>[2x]MDHLPIFCQLRDRDCLIVGGGDVAERKARLLLEAGARLTVNALTFIPQFTVWANEGMLTLVEGPFDETLLDSCWLAIAATDDDTVNQRVSDAAESRRIFCNVVDAPKAASFIMPSIIDRSPLMVAVSAGGTSPVLARLLREKLESLLPQHLGQVARYAGQLRARVKKQFATMGERRRFWEKFFVNDRLAQSLANADEKAVNATTERLFSEPLDHRGEVVLVGAGPGDAGLLTLKGLQQIQQADIVVYDRLVSDDIMNLVRADADRVFVGKRAGYHCVPQEEINQILLREAQKGKRVVRLKGGDPFIFGRGGEELETLCHAGIPFSVVPGITAASGCSAYSGIPLTHRDYAQSVRLVTGHLKTGGELDWENLAAEKQTLVFYMGLNQAATIQEKLIAFGMQADMPVALVENGTSVKQRVVHGVLTQLGELAQQVESPALIIVGRVVALRDKLNWFSNH

Siroheme is the modified isobacteriochlorin tetrapyrrole used by siroheme-dependent sulfite and nitrite reductases (SiR/NiRs) in catalyzing the six-electron reduction of sulfite to sulfide or nitrite to ammonia. CysG is encoded by a gene fusion between a C-terminal SUMT (CysGA) and an N-terminal bifunctional dehydrogenase/ferrochelatase (CysGB). The N-terminal enzyme module, CysGB, is a three-domain bifunctional dehydrogenase/ATP-independent class III ferrochelatase12 that performs the final two steps of siroheme biosynthesis. The C-terminal enzyme module, CysGA, is homologous to a well-studied class of SAM-dependent uro’gen III methyltransferases (SUMTs) that catalyzes the methylations to generate precorrin-210,13.

R260, which binds ring C C12 acetyl, and R261, which does not directly interact with carboxylate but contributes to the positively charged pocket that captures ring B, are part of the CysGA SUMT module. To test whether or not their contributions are essential for tetrapyrrole binding, we individually altered each to an alanine and tested the variants’ activities for dehydrogenase or chelatase activity. Both the R260A and R261A variants complement a cysG deficiency in E. coli grown on minimal media where SO42− is the sole sulfur source. The R261A variant has ~40-fold lower dehydrogenase activity and 20-fold lower chelatase activity. We next determined the X-ray crystal structures of the variants to test whether these alterations changed the relationship between the enzyme modules or their overall structure. Both R260A and R261A structures are similar to CysG and have a low root-mean-square deviation (RMSD) when aligned against Met8p14. R261 does not make a formal interaction with the tetrapyrrole, although it does contribute to the charged pocket that binds the carboxylates from ring B, so it is not surprising that removing the large, charged side chain does not substantially affect the structure. Interestingly, the culture expressing R260A, but not R261A, showed signs of precorrin-2 buildup in its pink fluorescence. R261A responded similarly to CysG to Co2+-challenged complementation, whereas R260A colonies were smaller and more strongly affected by increasing Co2+ concentration. R261A, D262A, and D262N retain some activity for both chemistries.> AMGQRAMKFCQGVVRELMSKKYASFNYPFLEPVDPVALNCPTYFDYVKEPMDLGTVSKKLSNWEYENLDQAEHDIRLIFQNCYAFN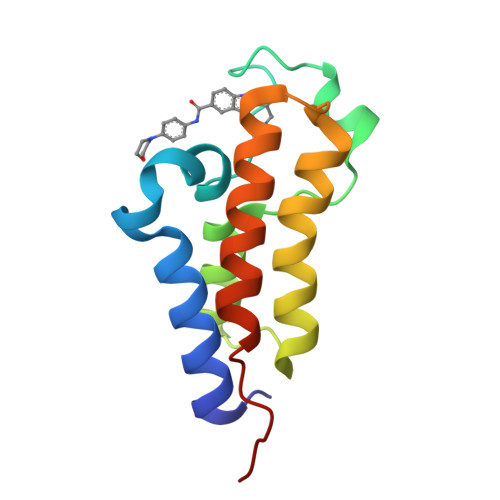PDGTIVNMMGHRLEDIFNTKWADRPLYSDVES>[2x]SGKIIGIDLGTTNSCVAIMDGTTPRVLENAEGDRTTPSIIAYTQDGETLVGQPAKRQAVTNPQNTLFAIKRLIGRRFQDEEVQRDVSIMPFKIIAADNGDAWVEVKGQKMAPPQISAEVLKKMKKTAEDYLGEPVTEAVITVPAYFNDAQRQATKDAGRIAGLEVKRIINEPTAAALAYGLDKGTGNRTIAVYDLGGGAFDISIIEIDEVDGEKTFEVLATNGDTHLGGEDFDSRLINYLVEEFKKDQGIDLRNDPLAMQRLKEAAEKAKIELSSAQQTDVNLPYITADATGPKHMNIKVTRAKLESL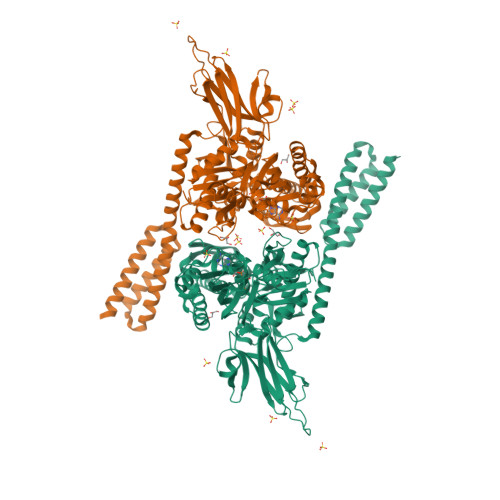VEDLVNRSIEPLKVALQDAGLSVSDIDDVILVGGQTRMPMVQKKVAEFFGKEPRKDVNPDEAVAIGAAVQGGVLTGDVKDVLLLDVTPLSLGIETMGGVMTTLIAKNTTIPTKHSQVFSMGGAVTIHVLQGERKRAADNKSLGQFNLDGINPAPRGMPQIEVTFDIDADGILHVSAKDKNSGKEQKITIKASSGLNEDEIQKMVRDAEANAEADRKFEELVQTRNQGDHLLHSTRKQVEEAGDKLPADDKTAIESALTALETALKGEDKAAIEAKMQELAQVSQKLMEIAQQQHAQQQHA> MISIMDRSEIVARENPVITQRVTNLLQTNAPLLFMPIDIHEVRYGAYTLFMYGSLENGYKAEVRIENIPVFFDVQIEFNDTNQLFLKSLLTAENIVYERLETLTQRPVMGYREKEKEFAPYIRIFFKSLYERRKAITYLNNMGYNTAADDTTCYYRMVSRELKLPLTSWIQLQHYSYEPRGLVHRFSVTPEDLVSYQNDGPTDHSIVMAYDIETYSPVKGTVPDPNQANDVVFMICMRIFWIHSTEPLASTCITMAPCKKSSEWTTILCSSEKNLLLSFAEQFSRWAPDICTGFNDSRYDWPFIVEKSMQHGILEEIFNKMSLFWHQKLDTILKCYYVKEKRVKISAEKSIISSFLHTPGCLPIDVRNMCMQLYPKAEKTSLKAFLENCGLDSKVDLPYHLMWKYYETRDSEKIADVAYYCIIDAQRCQDLLVRHNVIPDRREVGILSYTSLYDCIYYAGGHKVCNMLIAYAIHDEYGRIACSTIARGKREHGKYPGAFVIDPVKGLEQDKPTTGLDFASLYPSLIMAYNFSPEKFVASRDEANSLMAKGESLHYVSFHFNNRLVEGWFVRHNNVPDKMGLYPKVLIDLLNKRTALKQELKKLGEKKECIHESHPGFKELQFRHAMVDAKQKALKIFMNTFYGEAGNNLSPFFLLPLAGGVTSSGQYNLKLVYNFVINKGYGIKYGDTDSLYITCPDSLYTEVTDAYLNSQKTIKH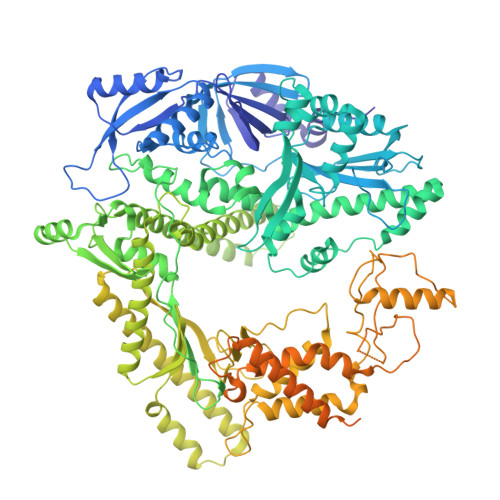YEQLCHEKVLLSMKAMSTLCAEVNEYLRQDNGTSYLRMAYEEVLFPVCFTGKKKYYGIAHVNTPNFNTKELFIRGIDIIKQGQTKLTKTIGTRIMEESMKLRRPEDHRPPLIEIVKTVLKDAVVNMKQWNFEDFIQTDAWRPDKDNKAVQIFMSRMHARREQLKKHGAAASQFAEPEPGERFSYVIVEKQVQFDIQGHRTDSSRKGDKMEYVSEAKAKNLPIDILFYINNYVLGLCARFINENEEFQPPDNVSNKDEYAQRRAKSYLQKFVQSIHPKDKSVIKQGNVHRQCYKYIHQEIKKKIGIFADLYKEFFNNTTNPIESFIQSTQFMIQYFDGEQKVNHSMKKMVEQHATASNRAGKPAGNPAGNALMRAIFTQLITEEKKIVQALYNKGDAIHDLLTYIINNINYKIATFQTKQMLTFEFSSTHVELLLKLNKTWLILAGIHVAKKHLQAFLDSYNNESPSRTFIQQAIEEECGSIKPSCYDFIS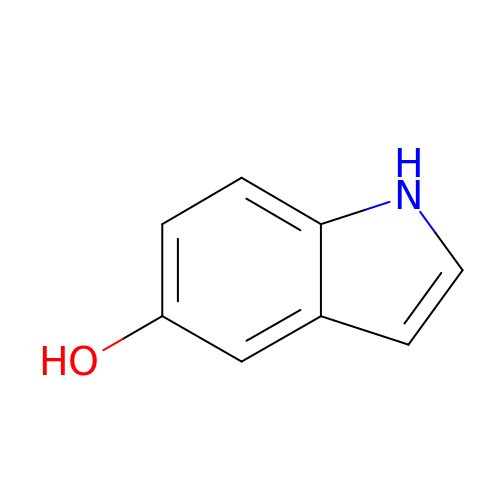1H-indol-5-ol | C8 H7 N O | LMIQERWZRIFWNZ-UHFFFAOYSA-N>[3x]MDTILLTGLFAAFFTTFAFAPQSIKTIRTRNTEGISVVMYIMFLTGVISWIAYGIMRSDFAVLIANIVTLFLAAPVLVITLINRRKKHVLESSGENLYFQ

The SWEETs mediate the facilitative diffusion of sugars, by allowing solute permeation across biological membranes down a concentration gradient. SWEETs possess seven transmembrane (TM) helices, consisting of a pair of 3TM repeats and an additional helix that spans the membrane to connect these two repeats, resulting in the ‘3+1+3’ arrangement of TM helices. Their bacterial homologues, the SemiSWEETs, have only three TM helices. Previous studies have shown that the SemiSWEETs assemble into dimers to function as sugar transporters, and thus they are considered to be an ancestral form of the SWEETs.

We crystallized EcSemiSWEET by the lipidic cubic phase (LCP) method and obtained crystals belonging to the space group P21212 (Crystal-I). The structure was determined by the Se-Met single-wavelength anomalous dispersion (Se-Met SAD) method and subsequently refined to 2.0 Å resolution against the data set from a native crystal. A total of six TM helices from two protomers create a central cavity that is widely open to the intracellular side. This cavity penetrates into the dimer core, but is completely occluded from the extracellular side and the lipid environment by the tight association of the extracellular regions and the surrounding TM helices, respectively. Hence, we designated this structure as the inward-open conformation. The high-resolution structure of Crystal-I revealed the presence of a monoolein molecule occupying the cavity of the inward-open state. The glycerol head group of the monoolein molecule is located in the pocket formed by symmetrically arranged residues in the dimer core. Within the pocket, the hydroxyl group of the glycerol head group forms direct and water-mediated hydrogen bonds with the side chains of Asn66. Given that glycerol and sugar share similar polyol moieties, the glycerol head group of the bound monoolein molecule is likely to be mimicking the sugar substrate. In the present structure in the inward-open conformation, the putative substrate-binding pocket is occupied by the monoolein molecule mimicking the substrate sugar, indicating that the observed structure represents an inward-open, substrate-binding state.>[3x]GLAEKLVPAKKVKNGVLYKSGHIKVSNVRCSYPHLDKPYGGEDGGEPKYSITLLMPKDTHGAIKKIIDEQIELTKKNHKTGALKVAPSMLFIKDGDVDFPDKPECEGMWVISARESTRPDVLNMEREELESPNEIAEEIYGGCWVSSVIRPWSQENKYGKRINANLLSVLKRKDDEPFGE

The hypothetical protein ORF6 of the Enc34 phage is conserved among all Nazgul-like phages and consists of a single domain, currently annotated as a domain of an unknown function DUF2815. Here, we present structural and functional characterization of the Enc34 ORF6 that allows us to establish its function as a single-stranded DNA-binding protein (SSB) and extend this annotation to other DUF2815 family members. The SSBs are ubiquitous within all kingdoms of life and in DNA viruses, and protect ssDNA intermediates during replication, repair and recombination. In this study, we show that the Enc34 ORF6 is structurally homologous to the gene 2.5 protein from bacteriophage T7, and present a high-resolution structure of ORF6 in complex with ssDNA, which reveals for the first time the structural basis for the ssDNA-binding mechanism of T7-type SSBs.

In T7 gp2.523 and T4 gp32, the removal of the acidic C-terminus results in higher affinity for DNA, and to further test the DNA binding properties of the Enc34 ORF6, a recombinant protein ORF6ΔC was constructed with the C-terminal 21 residues lacking. While the ssDNA-binding affinity of the truncated protein remained unchanged (bottom left), somewhat surprisingly, a similar affinity was observed also for dsDNA (bottom right). While co-crystallization attempts using the full-length protein were unsuccessful, the truncated ORF6ΔC protein could be crystallized both in absence of DNA and in presence of oligo-thymidine (dT). ORF6ΔC crystals without bound DNA diffracted to a slightly higher resolution (1.34 Å) than those of the full-length protein and had three molecules in the asymmetric unit. Due to different packing of loops and N-termini in the crystal, the three protein chains have Cα RMSDs of 0.8 to 1.1 Å when superimposed with the full-length ORF6.>MAIGIDKINFYVPKYYVDMAKLAEARQVDPNKFLIGIGQTEMAVSPVNQDIVSMGANAAKDIITDEDKKKIGMVIVATESAVDAAKAAAVQIHNLLGIQPFARCFEMKEACYAATPAIQLAKDYLATRPNEKVLVIATDTARYGLNSGGEPTQGAGAVAMVIAHNPSILALNEDAVAYTEDVYDFWRPTGHKYPLVDGALS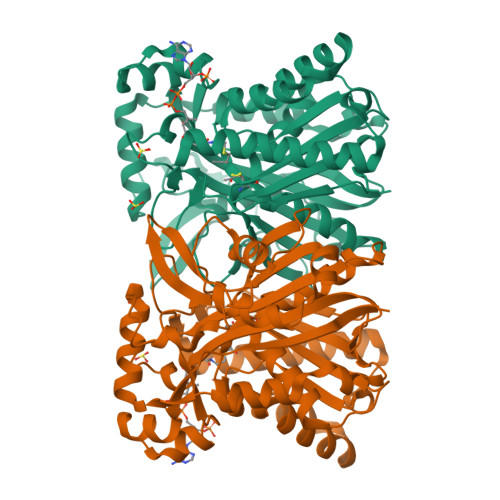KDAYIRSFQQSWNEYAKRQGKSLADFASLCFHVPFTKMGKKALESIIDNADETTQERLRSGYEDAVDYNRYVGNIYTGSLYLSLISLLENRDLQAGETIGLFSYGSGSVGEFYSATLVEGYKDHLDQAAHKALLNNRTEVSVDAYETFFKRFDDVEFDEEQDAVHEDRHIFYLSNIENNVREYHRPELEHHHHHH[4x]> DSVDYRKKGYVTPVKNQGQCGSCWAFSSVGALEGQLKKKTGKLLNLSPQNLVDCVSENDGCGGGYMTNAFQYVQKNRGIDSEDAYPYVGQEESCMYNPTGKAAKCRGYREIPEGNEKALKRAVARVGPVSVAIDASLTSFQFYSKGVYYDESCNSDNLNHAVLAVGYGIQKGNKHWIIKNSWGENWGNKGYILMARNKNNACGIA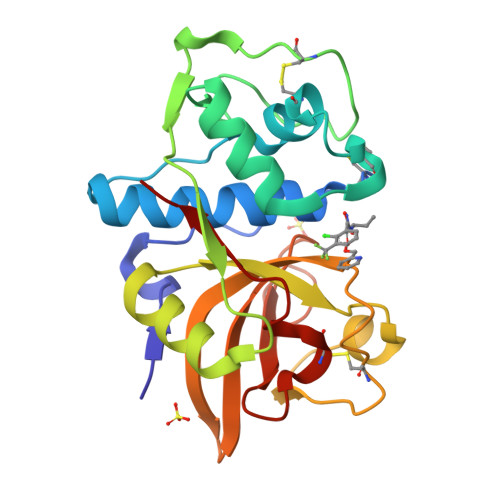NLASFPKM>GPKSSDHVDLPYNLTATKIDSDVFVVTDRDFYSSNVLVAKMLDGTVVIVSSPFENLGTQTLMDWVAKTMKPKKVVAINTHFHLDGTGGNEIYKKMGAETWSSDLTKQLRLEENKKDRIKAAEFYKNEDLKRRILSSHPVPADNVFDLKQGKVFSFSNELVEVSFPGPAHSPDNVVVYFPKKKLLFGGCMIKPK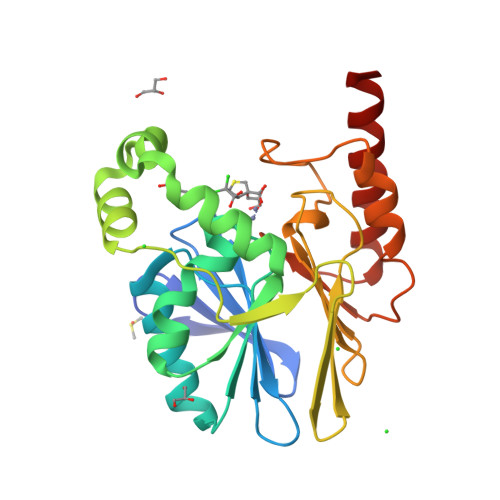ELGYLGDANVKAWPDSARRLKKFDAKIVIPGHGEWGGPEMVNKTIKVAEKAVGEMRL[2x]(3Z)-3-[(4-{[2-(dimethylamino)ethyl]carbamoyl}-3,5-dimethyl-1H-pyrrol-2-yl)methylidene]-2-oxo-N-[(1R)-1-phenylethyl]-3,7-dihydro-2H-indole-5-carboxamide 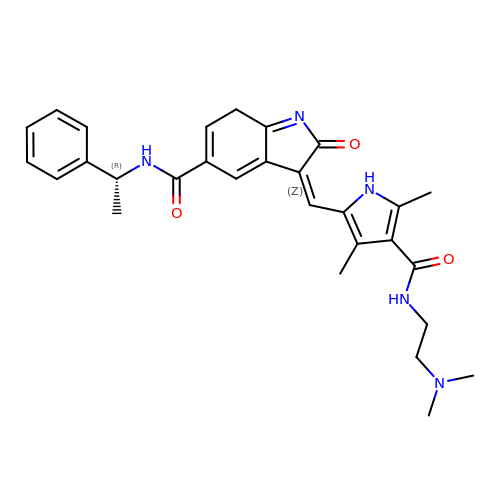| C29 H33 N5 O3 | HKWYOXJKRXXECG-MPGAHLTBSA-N4-[(3~{R},4~{S})-2-oxidanylidene-3,4-diphenyl-azetidin-1-yl]piperidine-1-carbaldehyde 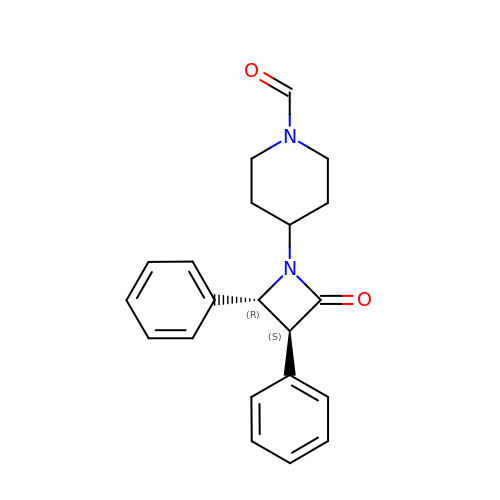| C21 H22 N2 O2 | DIWMCVCOMCANGI-UXHICEINSA-N> GSHMPTVEELYRNYGILADATEQVGQHKDAYQVILDGVKGGTKEKRLAAQFIPKFFKHFPELADSAINAQLDLCEDEDVSIRRQAIKELPQFATGENLPRVADILTQLLQTDDSAEFNLVNNALLSIFKMDAKGTLGGLFSQILQGEDIVRERAIKFLSTKLKTLPDEVLTKEVEELILTESKKVLEDVTGEEFV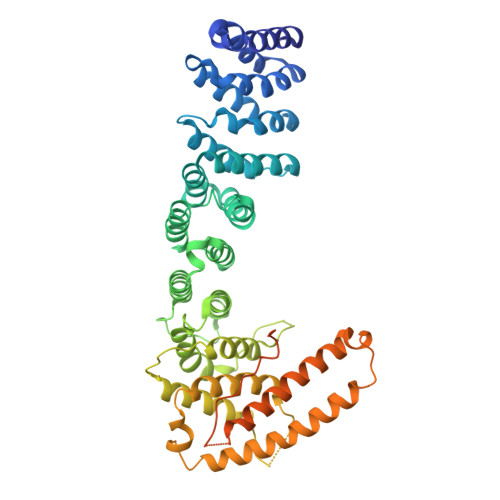LFMKILSGLKSLQTVSGRQQLVELVAEQADLEQTFNPSDPDCVDRLLQCTRQAVPLFSKNVHSTRFVTYFCEQVLPNLGTLTTPVEGLDIQLEVLKLLAEMSSFCGDMEKLETNLRKLFDKLLEYMPLPPEEAENGENAGNEEPKLQFSYVECLLYSFHQLGRKLPDFLTAKLNAEKLKDFKIRLQYFARGLQVYIRQLRLALQGKTGEALKTEENKIKVVALKITNNINVLIKDLFHIPPSYKSTVTLSWKPVQKVEIGQKRASEDTTSGSPPKKSSAGPKRDARQIYNPPSGKYSSNLGNFNYERSLQGK>[3x]ATAAEIAALPRQKVELVDPPFVHAHSQVAEGGPKVVEFTMVIEEKKIVIDDAGTEVHAMAFNGTVPGPLMVVHQDDYLELTLINPETNTLMH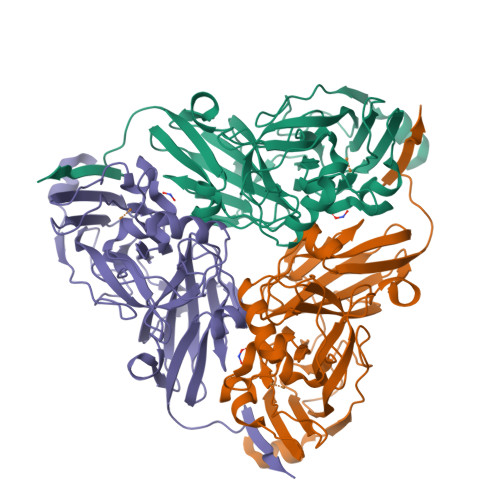NIDFHAATGALGGGGLTEINPGEKTILRFKATKPGVFVYHCAPPGMVPWHVVSGMNGAIMVLPREGLHDGKGKALTYDKIYYVGEQDFYVPRDENGKYKKYEAPGDAYEDTVKVMRTLTPTHVVFNGAVGALTGDKAMTAAVGEKVLIVHSQANRDTRPNLIGGHGDYVWATGKFNTPPDVDQETWFIPGGAAGAAFYTFQQPGIYAYVNHNLIEAFELGAAAHFKVTGEWNDDLMTSVLAPSGTIEGR>[2x]CDLNINDDPNYPMNDQVTADLIFPSISASIASAVGGEIYNYAGFFAQYYEQKPESNQYNTLCEYTFTESSQQMDYSYRILFAGALEDAKQVLEKTTNPADRFATTILRAYAFQIMVDNTSDSPYSEALQGNANATPKWDTGETVYKGILGEIDAAEAALDGSGMDVPDLIFNKNIAQWKGFANALRLRMYLRFIDANIDAASYTEKVKTLVQNNEFFTGDVKLDCFLDETDKRNPWYNTNAVGLTGNHCAAYPLVSYLSSTGDPRIAYGISKTDADGKYVGQLPGGKTHMQSILGTDNWKNKNVSAIDYSIGATKPVYFFTQAELQFLIAEVYARFHNDDANAKSAYEAGVTADFAV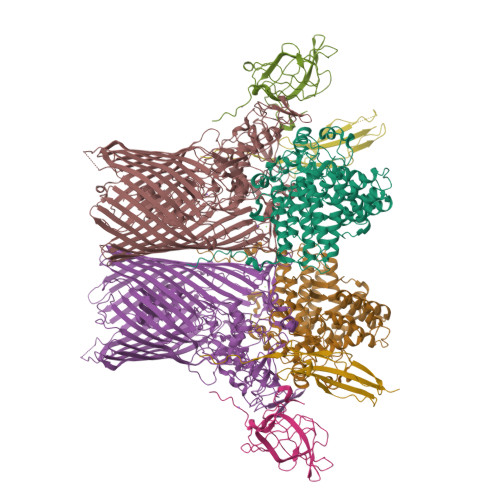RGFAGQENTILEGACAWSAASTQADKLNLIYMQKWVSLFYMDHMEAWSEIRRTDCPKLSSYSAAQIQASESVYTPGELVAPWTNGLEAGGLMKRMTYPLSARQQNVNTPAGVPGSTPVWWDIK;>[2x]MQTQEVAIKPNLKVVLRSDAQQIDEVVVTAMGIKRSEKALGYAATSVGGEKIAESRTSDVMSSLAGKIAGVQISSTSSDPGASNSVIIRGVSSLSGTNQPLYVVDGVPLNNSTVYSTDGLNSGYDFGNGANAINPDDVANMTILKGAAATALYGSRAANGVVMITTKSGRKEKGVGIEYNGGVQWSTVLRLPEFQNEFGMGWNGNHTELENGSWGPRFDGSMQLWGNVYNNSQKLKPYVAMPDNIKDFFDAGFRYSNSLSFNGATDKSDYYVSFSQISDDGMIPTDADSYDKYTFSARGSHKAGALTFSSSLNYAYQKNNFATTGQGLSMLNSLYQTPRDISIIGLEDQNDPFNTPGYYYTPYGVMNPYYILNNYLNEYESERFYGKFQLDYEFLKYFKFTYRMGLDTTTGQSDKGKPNLYALYYEGTPNGEGQGSSSPFSGETGQYSEQITRRREINQDIMVNFNMPVNDFNINALVGFNGNERKVSYQYSEVNDLTIPTWFNLKNSGKTPIVEQHMELRRLMGVFGQFEGSWKNMLYLTVTARNDWSSTLPKENRSFFYPGITGSFIFSELLNDNLQDVITFGKIRASWGKTGNDADVYMVNPVYAQSSNRIPFGSLTFPLGGVNAYSAGNVLGSNTLSPEMTTESEVGLNMAFFKNRLSFDVSYYNRNTDKQIFSLAMDPASGYTAQNMNLGKIRNRGIELLISGTPIRTKDFSWELTWNFTKNWSKVISLPEELGGITTIYGLNGGTSMYAITGMPVGVFKAQVAERDPQGRIVVNSSTGLPVEASEFGICGDMNNKYQMGVSTNLKYKGISLGIDFDIRQGGVMYSRTKDINYFTGNAIQTAYNDRNPLIVPNSVNKIVNGENVTYVENTTPITSSNIYKYWGDGGSDMGSCFLVDKSYVKLRSVVLGWDLPKRWLAKTPFQAVKVSAYGNNLFVWTPSSNTFIDPEMTSFGNDLEGNYGEYTANPSSRRFGFNLMVKF;>CDNDTEPGGTAVEKMAGDWWVTVNAFIDGKEVEDPFGAGHLQMSTYNTASNSETEMWLDDLGNFWEYKLKVNVNYAARTFSTTGFVDNVTYESKVKITDGKVLEKAATTPSGMPADSIVYMVQFDDDEDGLTYKVSGFRRTGFPADDF[2x];>[2x]CDKSTDDTSKVTYFVTLEREGDEKIVLEKGQPFVEPGYYAEMNGEDITESVQIKGSVDVNTPGIYNLVYAAYNEDGFAKTFTRTVYVADNTASPLKSGIYTVAEGSKRTAPSVVAFSGYEIVIFQMEPGIFYISDFLGGWYDQRAGYGPDYAMVGKFELNDDNTITPLESYVAGWGDSMDQMTNTLLDPATGTLKWTVAYAGQLSFDIIVKQ;>GGGGGGGGGG[2x]> FEKAPDSVPETITGGRYSLKDGYYVYLDKQGKQVVGPKNIDNHLQYFDETTGKQVKGDFRSVNGKRIYFNANLGYADDYTTDVAGKLVGYDSNGNQVKAGYVTNSQGKTYYFNNQGEAIIGLKTDNNKTQYFGPDGAQVKGAFQQVNGKNIYFDAQTGYARQNVGFLDGTAKGFDEQGNQIKSGIATDLSGNVYYFDASGKMLTGVQNIDGKKYYFDEQGHRRRNYAGVFNNEFIYFGLDGVGQSAIEYQFEKGLTSQNSVATSHNAAKSYDTKSFTNVDGFLTANSWYRPTDILRNGTKWEPSTETDFRPLLMTWWPDKEVQANYLNYMSALGLGDQKIYTGASSQLDLNNAALIVQEAIEKKISLEKSTKWLDDSIKSFIKSKRKDIQGNLVDTNPGWTIDSETGSTNHLQNGAFIFTNSPLVPEANAAEGNRLINRTPSQQTGNHISYASQPYSGDDWGYELLLGNDVDNSNPIVQAEQLNWIHYLMNFGTITAPQDPDAHLANFDSIRIDAVDNVDADLLQIAGDYFKAAYQVGENDKNANQHIHILQDWSPNDVWYNQQVNGNSQLTMDATMQNQLLASLTRPITSRDSMKSFTKDALLVHRTADNSYNQAVPNYSFIRAHDSEVQTIIAKIISDKHPDLYPTVDKALLAKDSALYDEAFTEYNADMQKISSQKQYTHNNMPSAYAILLTNKDTVPRVYYGDLFTDNGEYMANKTPYYDAITSLLTARTKFVSGGQSLSVDKNDVLTSVRYGKGALSATDNGSSDTRNQGI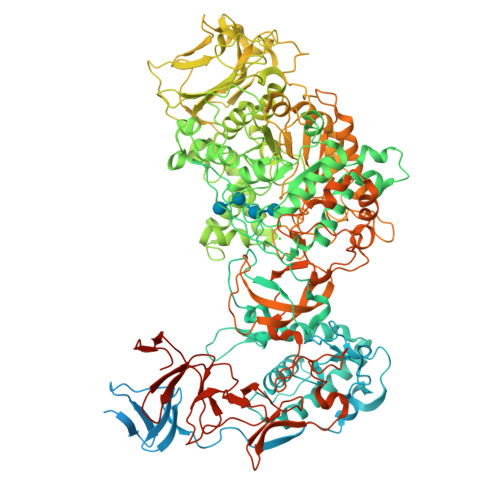GVIVSNNPNLDLNNDKVTLSMGISHAHQAYRPLLLTNSQGIVAYATDSEVPQNLYKTTNDKGELTFDASEIKGYDTVQTSGYLAVWVPVGASDEQDARTIASTEKNNGNSVYHSNAALDSQLIYEGFSNFQTVPSKNASADEYANVIIAKHAADFNKWGVTSFQMAPQYRSSTDGSFLDAVDTVQNGYAFTDRYDLGFNAADGSKNPTKYGTDEDLRNAIKSLHAQKTYDGSSIQVMADFVPDQLYNMPLEQAVSVIRTDKYGVNSENPDIQNIIYAANIKSSGTDYQSIYGGKYLAELQKNPLFKSLFDRIQISTKKTIDPNTRITQWSAKYFNGSNIQGKGINYVLKDWASNKYFNVSSNDDMYSRLPKQLMNQESNTGFIVDDIGVKYYSISGYQAKNTFVEDGNGEWYYFDNDGYMVKSTEESGPLRTVNASSKKYYILPNGVEIRNSFGQDIQGNTYYFDARGEMVTSQYISDDTQNIYYFNNDGTMAKKGGRADPAFLYKVVHHHHHH>[2x]MEGLAGYVYKAASEGKVLTLAALLLNRSESDIRYLLGYVSQQGGQRSTPLIIAARNGHAKVVRLLLEHYRVQTQQTGTVRFDGYVIDGATALWCAAGAGHFEVVKLLVSHGANVNHTTVTNSTPLRAACFDGRLDIVKYLVENNANISIANKYDNTCLMIAAYKGHTDVVRYLLEQRADPNAKAHCGATALHFAAEAGHIDIVKELIKWRAAIVVNGHG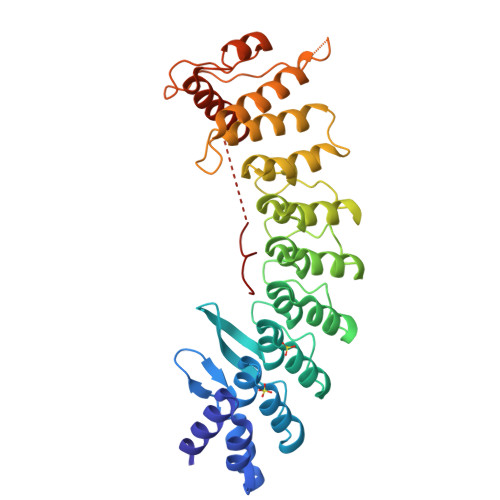MTPLKVAAESCKADVVELLLSHADCDRRSRIEALELLGASFANDRENYDIIKTYHYLYLAMLERFQDGDNILEKEVLPPIHAYGNRTECRNPQELESIRQDRDALHMEGLIVRERILGADNIDVSHPIIYRGAVYAD Type III CRISPR systems are innate immune systems found in bacteria and archaea, which produce cyclic oligoadenylate (cOA) second messengers in response to viral infections. In these systems, Csm6 proteins serve as ancillary nucleases that degrade single-stranded RNA (ssRNA) upon activation by cOA. In addition, Csm6 proteins also possess cOA-degrading activity as an intrinsic off-switch to avoid degradation of host RNA and DNA that would eventually lead to cell dormancy or cell death. The two TtCsm6 monomers dimerize in an X-shape, and each monomer contains an N-terminal CARF domain, an intermediate helix-turn-helix (HTH) domain and a C-terminal HEPN domain.

Guided by this structure, we then identified a TtCsm6 variant Y161A, which displays a sustained cA4-activated RNase activity without cleaving cA4. We next co-crystallized TtCsm6Y161A with cA4 and determined the structure at a resolution of 2.9 Å. As expected, we observed a cA4 molecule binding in the CARF domain, which remains uncleaved as evidenced by its unambiguous electron density, indicating that the structure was determined in the pre-cleavage state. One significant variation is that, in this cA4-bound structure, we were able to observe the coordination of both the scissile phosphate and the 2ˊ-OH nucleophile, which are positioned by S60 and T59, respectively, resulting in an O2ˊ-P-O5ˊ angle of 159o. Furthermore, the contact of nonscissile phosphate with Y161 is abrogated due to the alanine substitution. Upon cA4 binding, the primary conformational change occurs in the CARF domain, where a mobile loop along with the two helices situated above the catalytic center switch from an open to a closed conformation, completely enclosing the cA4 molecule within the catalytic center. In the cA4-bound structure, the HTH domains of the two monomers move toward each other with a maximum shift of ~10 Å compared to the apo state (Movie EV1). However, in the cA4-bound structure, the hydrogen bonds between N416 and H422 are disrupted, causing them to separate with each other by a maximum distance of 9.4 Å. Moreover, R415 also disassociates from E332 and exposes its guanidine side chain to the surface of catalytic center. This remodeling positions the R-X4-6-H motif into a catalytically competent conformation.

>[2x]EDLDALWERYREAVRAGGNPQALYQEMVWPALLALWREKPRVYPFPQAFAVSVHTLGTSPEATALAILGAGAERVYVLHTPESARFLPRLRQDTGKDLYPVEIGKSDVEAIYREVKRLLEKHPEVPVALDLTSGTKAMSAGLAAAGFFFQRFYPKVRVVAVDNEDYDPELRRPRAGTEKLRILPNPHEALAEVDALFAKELYGKGEFGQAAAYFRGMVGRTGNQAYALYALLAEMYRAWRALDFGEALKAGRKLLGQLSQNVWLNHPLNARREALEAQVALLEAVDRFLKARDFALKEGVYGLARTLLHLAQEAKEEAAVLAALYAYRALELLLQERLALLGRRAEAPGLSPEEAEALRKALAELLGVLPEEVRLPAKLGLLDLLAFLRLKGDEALGRLSLAELRGLAGALKGRNSALLVHGFDVPSPKAVEGIARLAQGLLQDLEARTALGPLSPEPVPLGF>MAASLPSTLSFSSAPDEIQHPQIKFSEWKFKLFRVRSFEKAPEEAQKEKDSSEGKPYLEQSPVVPEKPGGQNSILTQRALKLHPKFSKKFHADGKSSDKAVHQARLRHFCRICGNRFKSDGHSRRYPVHGPVDAKTQSLFRKKEKRVTSWPDLIARIFRIDVKADVDSIHPTEFCHDCWSIMHRKFSSSHSQVYFPRKVTVEWHPHTPSCDICFTAHRGLKRKRHQPNVQLSKKLKTVLNHARRDRRKRTQARVSSKEVLKKISNCSKIHLSTKLLAVDFPAHFVKSISCQICEHILADPVETSCKHLFCRICILRCLKVMGSYCPSCRYPCFPTDLESPVKSFLNILNSLMVKCPAQDCNEEVSLEKYNHHVSSHKESKETLVHINKGGRPRQHLLSLTRRAQKHRLRELKIQVKEFADKEEGGDVKAVCLTLFLLALRARNEHRQADELEAIMQGRGSGLQPAVCLAIRVNTFLSCSQYHKMYRTVKAITGRQIFQPLHALRNAEKVLLPGYHPFEWQPPLKNVSSRTDVGIIDGLSGLASSVDEYPVDTIAKRFRYDSALVSALMDMEEDILEGMRSQDLDDYLNGPFTVVVKESCDGMGDVSEKHGSGPAVPEKAVRFSFTVMRITIEHGSQNVKVFEEPKPNSELCCKPLCLMLADESDHETLTAILSPLIAEREAMKSSELTLEMGGIPRTFKFIFRGTGYDEKLVREVEGLEASGSVYICTLCDTTRLEASQNLVFHSITRSHAENLQRYEVWRSNPYHESVEELRDRVKGVSAKPFIETVPSIDALHCDIGNAAEFYKIFQLEIGEVYKHPNASKEERKRWQATLDKHLRKRMNLKPIMRMNGNFARKLMTQETVDAVCELIPSEERHEALRELMDLYLKMKPVWRSSCPAKECPESLCQYSFNSQRFAELLSTKFKYRYEGKITNYFHKTLAHVPEIIERDGSIGAWASEGNQSGNKLFRRFRKMNARQSKCYEMEDVLKHHWLYTSKYLQKFMNAHNALKSSGFTMNSKETLGDPLGIEDSLESQDSMEF[2x];>[2x]MSLQMVTVGHNIALIQPGFSLMNFDGQVFFFGQKGWPKRSCPTGVFHFDIKQNHLKLKPAIFSKDSCYLPPLRYPATCSYKGSIDSDKHQYIIHGGKTPNNELSDKIYIMSVACKNNKKVTFRCTEKDLVGDVPEPRYGHSIDVVYSRGKSMGVLFGGRSYMPSTQRTTEKWNSVADCLPHVFLIDFEFGCAT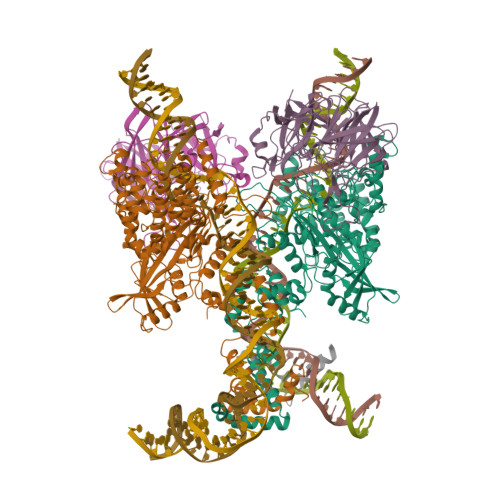SYILPELQDGLSFHVSIARNDTVYILGGHSLASNIRPANLYRIRVDLPLGTPAVNCTVLPGGISVSSAILTQTNNDEFVIVGGYQLENQKRMVCSLVSLGDNTIEISEMETPDWTSDIKHSKIWFGSNMGNGTIFLGIPGDNKQAMSEAFYFYTLRCSEEDLSEDQKIVSNSQTSTEDPGDSTPFEDSEEFCFSAEATSFDGDDEFDTYNEDDEDDESVTGYWITCCPTCDVDINTWVPFYSTELNKPAMIYCSHGDGHWVHAQCMDLEERTLIHLSEGSNKYYCNEHVQIARALQTPKRNPPLQKPPMKSLHKKGSGKVLTPAKKSFLRRLFD;> MGKGDPKKPRGKMSSYAFFVQTCREEHKKKHPDASVNFSEFSKKCSERWKTMSAKEKGKFEDMAKADKARYEREMKTYIPPKGETKKKFKDPNAPKRPPSAFFLFCSEYRPKIKGEHPGLSIGDVAKKLGEMWNNTAADDKQPYEKKAAKLKEKYEKDIAAYR> SVLSDFQEAVPTVVGIPDGTAVVGRSFRVSIPTDLIASSGEIIKVSAAGKEALPSWLHWDPHSHILEGLPLDTDKGVHYISVSAARLGANGSHVPQTSSVFSIEVYPEDHNEPQSVHAASSDPGEVVPSACAADEPVTVLMVILDADLTKMTPKQRIDLLNRMQSFSEVELHNMKLVPVVNNRLFDMSAFMAGPGNAKKVVENGALLS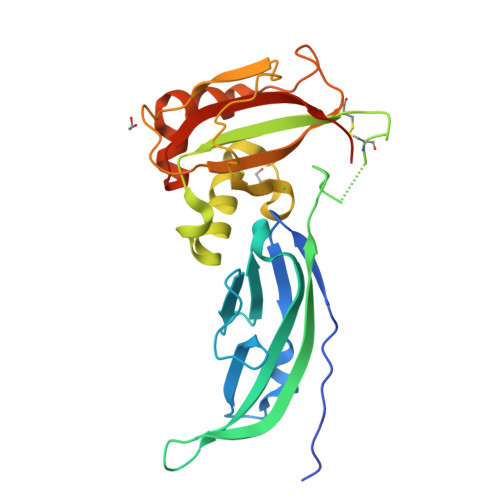WKLGCSLNQNSVPDIRGVETPAREGAMSAQLGYPVVGWHIANKKPTLPKRLRRQIH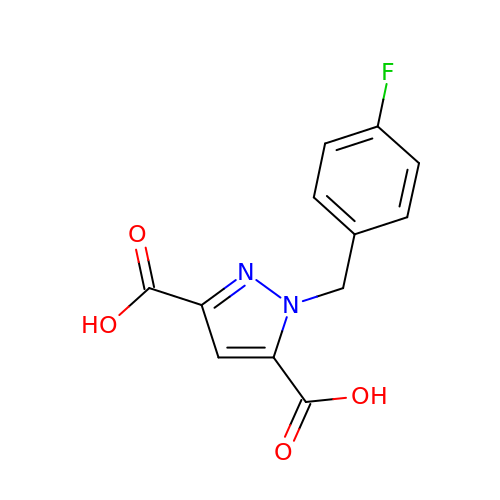1-[(4-fluorophenyl)methyl]pyrazole-3,5-dicarboxylic acid | C12 H9 F N2 O4 | YYCGCLWGMQYTDZ-UHFFFAOYSA-N> SCSKCRKEMGQVEI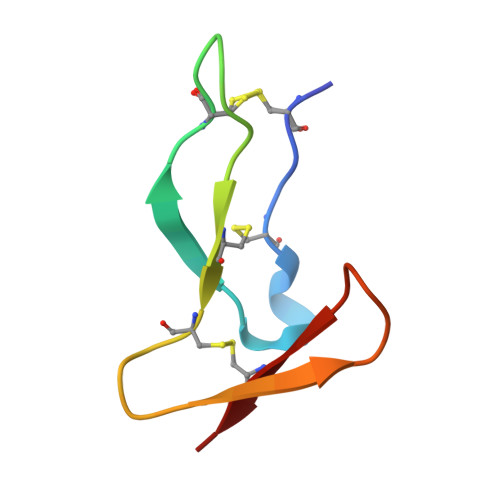SSCTVDRDTVCGCRKNQYRHYWSENLFQCFN> MQVSLPREDTVYIGGALWGPATTWNLYAPQSTWGTDQFMYLPAFQYDLGRDAWIPVIAERYEFVDDKTLRIYIRPEARWSDGVPITADDFVYALELTKELGIGPGGGWDTYIEYVKAVDTKVVEFKAKEENLNYFQFLSYSLGAQPMPKHVYERIRAQMNIKD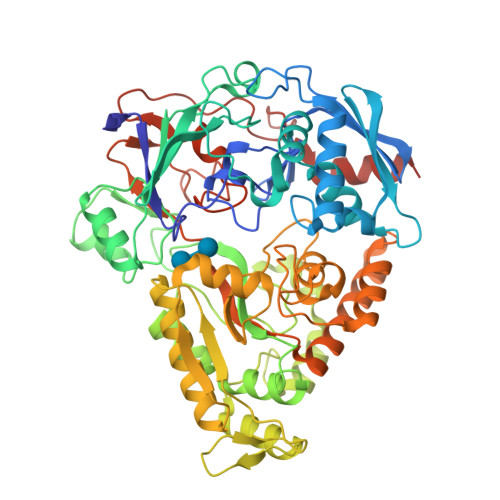WINDKPEEQVVSGPYKLYYYDPNIVVYQRVDDWWGKDIFGLPRPKYLAHVIYKDNPSASLAFERGDIDWNGLFIPSVWELWEKKGLPVGTWYKKEPYFIPDGVGFVYVNNTKPGLSDPAVRKAIAYAIPYNEMLKKAYFGYGSQAHPSMVIDLFEPYKQYIDYELAKKTFGTEDGRIPFDLDMANKILDEAGYKKGPDGVRVGPDGTKLGPYTISVPYGWTDWMMMCEMIAKNLRSIGIDVKTEFPDFSVWADRMTKGTFDLIISWSVGPSFDHPFNIYRFVLDKRLSKPVGEVTWAGDWERYDNDEVVELLDKAVSTLDPEVRKQAYFRIQQIIYRDMPSIPAFYTAHWYEYSTKYWINWPSEDNPAWFRPSPWHADAWPTLFIISKKSDPQPVPSWLGTVDEGGIEIPTAKIFEDLQKATMHHHHHH5-HYDROXYLAEVULINIC ACID | C5 H10 O3 | 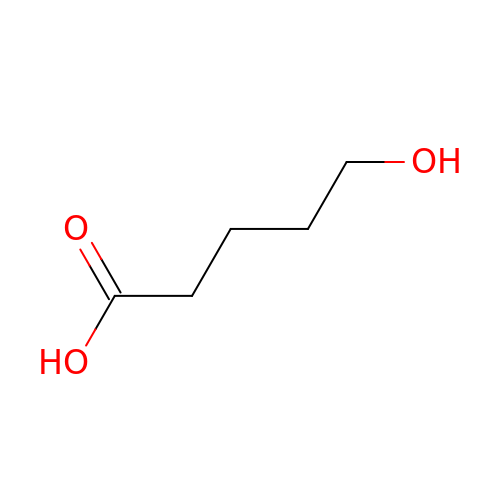PHOJOSOUIAQEDH-UHFFFAOYSA-N> RRASRFAQWAIHPTFNLKSLSCSLEVSKDSRTVT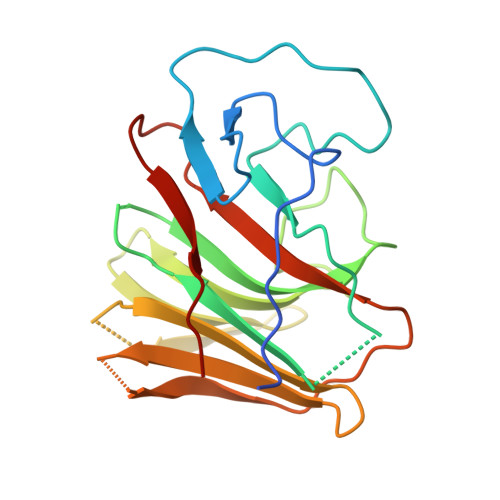VSHRPQPYRWSCERFSTSQVLCSQALSSGKHYWEVDTRNCSHWAVGVASWEMSRDQVLGRTMDSCCVEWKGTSQLSAWHMVKETVLGSDRPGVVGIWLNLEEGKLAFYSVDNQEKLLYECTISASSPLYPAFWLYGLHPGNYLIIKQVKV>IVGGYECRKNSASYQASLQS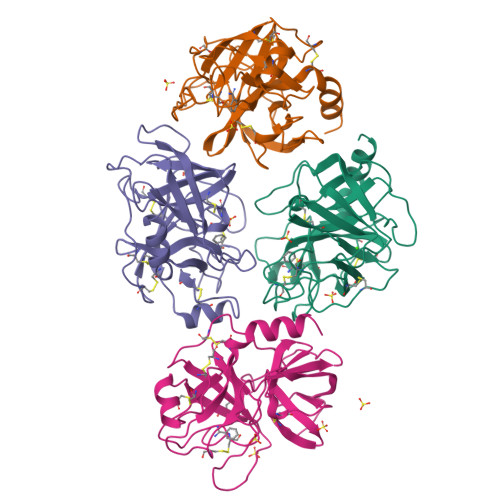GYHFCGGSLISSTWVVSAAHCYKSRIQVRLGEHNIAVNEGTEQFIDSVKVIMHPSYNSRNLDNDIMLIKLSKPASLNSYVSTVALPSSCASSGTRCLVSGWGNLSGSSSNYPDTLRCLDLPILSSSSCNSAYPGQITSNMFCAGFMEGGKDSCQGDSGGPVVCNGQLQGVVSWGYGCAQRNKPGVYTKVCNYRSWISSTMSSN[4x]> MKRIYIFLLCFAVLLPVGGKTAQAKEQAGEQYLLLEHVKDKSKLLDTAEQFHIHADVIEEIGFAKVTGEKQK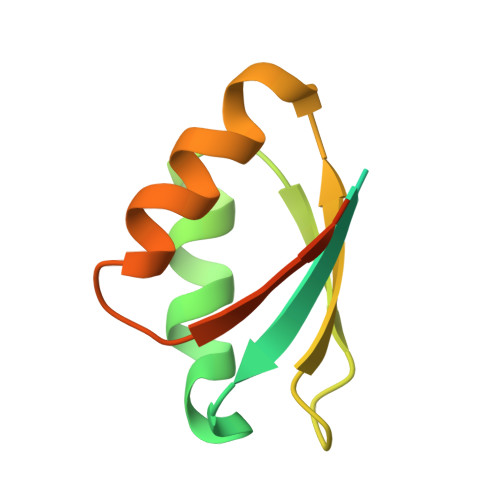LAPFTKKLAEKVGADVIEKPIANTAVNE N-(4-hydroxy-2,6-dimethylphenyl)-4-methoxybenzenesulfonamide 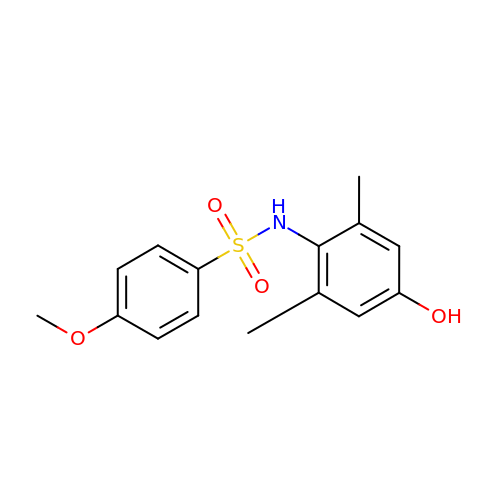| C15 H17 N O4 S | UXSFANIQULVRMS-UHFFFAOYSA-N>[2x]MCAQYCISFADVEKAHINIRDSIHLTPVLTSSILNQLTG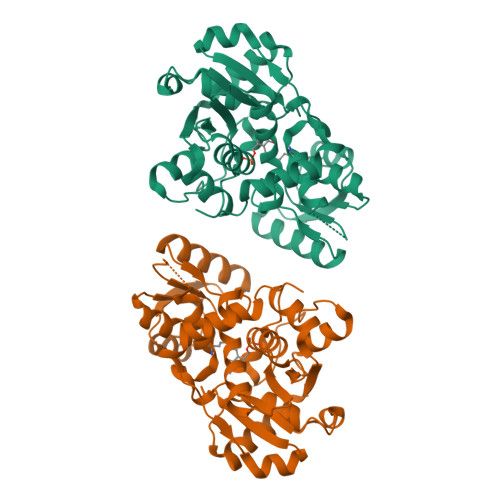RNLFFKCELFQKTGSFKIRGALNAVRSLVPDALERKPKAVVTHSSGNHGQALTYAAKLEGIPAYIVVPQTAPDCKKLAIQAYGASIVYCEPSDESRENVAKRVTEETEGIMVHPNQEPAVIAGQGTIALEVLNQVPLVDALVVPVGGGGMLAGIAITVKALKPSVKVYAAEPSNADDCYQSKLKGKLMPNLYPPETIADGVKSSIGLNTWPIIRDLVDDIFTVTEDEIKCATQLVWERMKLLIEPTAGVGVAAVLSQHFQTVSPEVKNICIVLSGGNVDLTSSITWVKQAERPASYQSVSVLEHHHHHH>EVFLKFVILHAEDDTDEALRVQNLLQDDFGIKPGIIFAEMPCG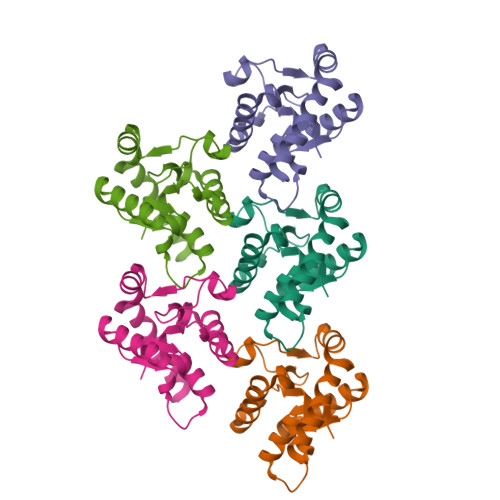RQHLQNLDDAVNGSAWTILLLTENFLRDTWCNFQFYTSLMNSVNRQHKYNSVIPMRPLNNPLPRERTPFALQTINALEEESRGFPTQVERIFQESVYKTQQTIWKETRNMVQR[5x]> MGSSHHHHHHPFTIDSARGIFPNTLAADVVPATIARFSQLNAEDQLALIWFAYLEMGKTLTIAAPGAASMQLAENALKEIQAMGPLQQTQAMCDLANRADTPLCRTYASWSPNIKLGFWYRLGELMEQGFVAPIPAGYQLSANANAVLATIQGLESGQQITVLRNAVVDMGFTAGKDGKRIAEPVVPPQDTASRTKVSIEGVTNATVLNYMDNLNANDFDTLIELFTSDGALQPPFQRPIVGKENVLRFFRE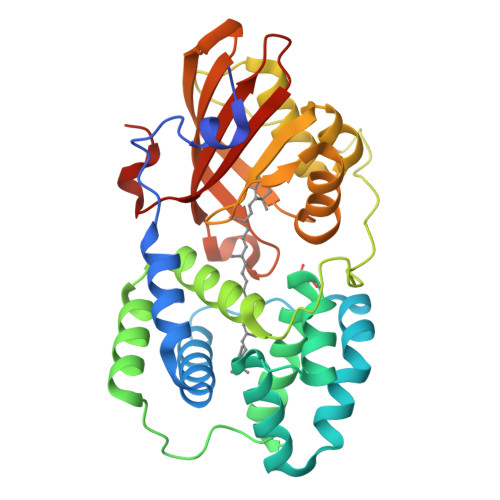ECQNLKLIPERGVTEPAEDGFTQIKVTGKVQTPWFGGNVGMNIAWRFLLNPEGKIFFVAIDLLASPKELLNFAR3-bromo-3-oxopropanoic acid | C3 H3 Br O3 | 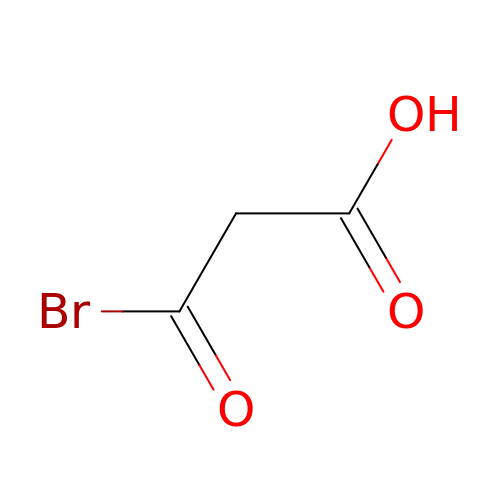RSZXDOPLBKMETA-UHFFFAOYSA-N> GSGSMETLCQRLNVCQDKILTHYENDSTDLRDHIDYWKHMRLECAIYYKAREMGFKHINHQVVPTLAVSKNKALQAIELQLTLETIYNSQYSNEKWTLQDVSLEVYLTAPTGCIKKHGYTVEVQFDGDICNTMHYTNWTHIYICEEASVTVVEGQ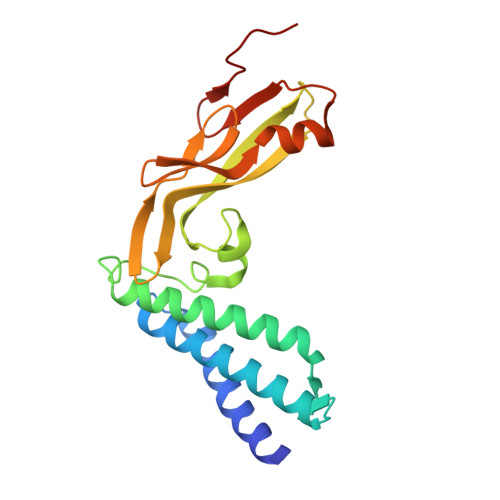VDYYGLYYVHEGIRTYFVQFKDDAEKYSKNKVWEVHAGGQVILCPTSVFS>ETGCKPEYYYAIAKNDRIGPLGAEGLTTVWKDYSPEMTLEDTMVIASCRDGKFMYLSRCTRETRYLAILHSRALPTSVVFKKLFEGQKQGDTVEMDDDFEFGLCPCDAKPIVRGKYNTTLLNGPAFQMVCPIGWTGTVSCMLANRDTLDTAVVRTYRRSRPFPYRQGCITQKVLGEDLYDCILGGNWTCVTG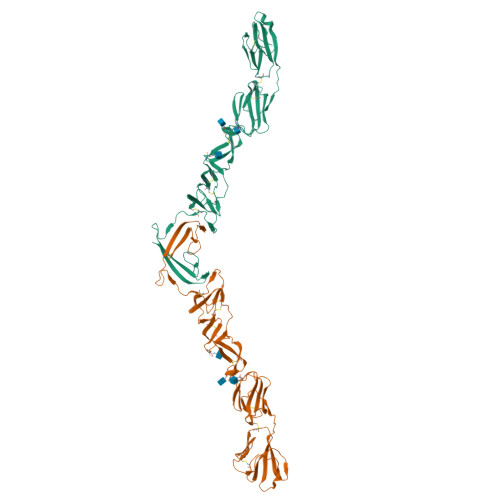DQLQYSGGSIESCKWCGFKFQRSEGLPHYPIGKCRLKNETGYRLVDNTSCNREGVAIVPQGTVKCKIGDTTVQVIALDTKLGPMPCKPYEIISSEGPVEKTACTFNYTKTLKNKYFEPRDSYFQQYMLKGEYQYWFDLEVTDGTK[2x]>[2x]MGKLFGTDGVRGIVNKELTPELVLKLSKAIGTFFGKNSKILVGRDVRAGGDMLVKIVEGGLLSVGV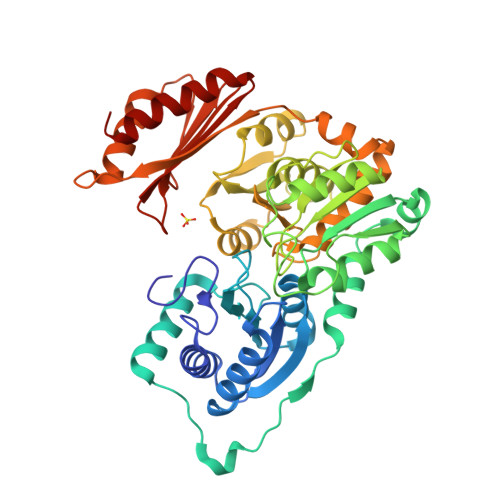EVYDGGMAPTPALQYAVKTLGYDGGVVITASHNPAPYNGIKVVDKDGIEIRREKENEIEDLFFTERFNTIEWSSLTTEVKREDRVISTYVNGILSHVDIEKIKKKNYKVLIDPANSVGALSTPLVARALGCKIYTINGNLDPLFSARQPEPTFDSLKETAEVVKTLKVDLGVAHDGDADRAIFIDSEGRVQWGDRSGTLLSYWASVKNPKAIKKIVTAVSSSSLVEEYLSKYNIQVDWTKVGSVDIAHKVADENALAGFEENGGFMYPPHQYVRDGAMSFALMLELLANENVSSAELFDRLPKYYLVKTKVDLKPGLMVEEIYKKILEVYSTSSVKAITIDGVKIIGKDFWFLVRKSGTEPIIRIMAEAKDENVANNLVNELKKIVEGK> GSHMDPLSNFEHKVITECVTIVLGDAIQVAKCYGESVLVNAANTHLKHGGGIAGAINAASKGAVQKESDEYILAKGPLQVGDSVLLQGHSLAKNILHVVGPDARAKQDVSLLSKCYKAMNAYPLVVTPLVSAGIFGVKPAV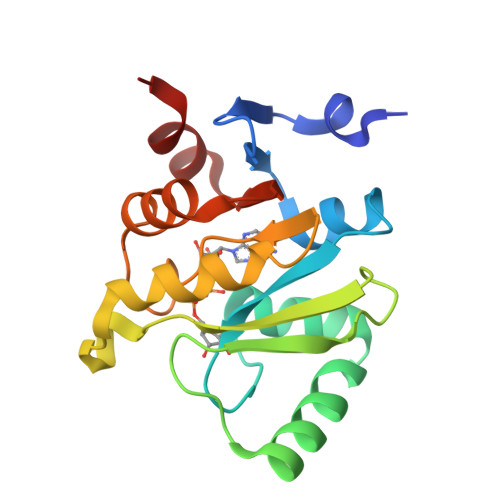SFDYLIREAKTRVLVVVNSQDVYKSLTIVD>[2x]MTDDKKKGKFIVFEGLDRSGKSTQSKLLVEYLKNNNVEVKHLYFPNRETGIGQIISKYLKMENSMSNE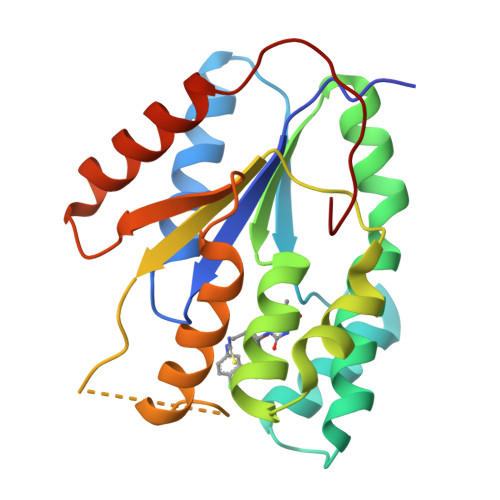TIHLLFSANRWEHMNEIKSLLLKGIWVVCDRYAYSGVAYSSGALNLNKTWCMNPDQGLIKPDVVFYLNVPPNYAQNRSDYGEEIYEKVETQKKIYETYKHFAHEDYWINIDATRKIEDIHNDIVKEVTKIKVEPEEFNFLWS Here, we show that AGE crosslinking is harnessed to activate an antibacterial phospholipase effector protein deployed by the type VI secretion system of Enterobacter cloacae. Endogenous methylglyoxal reacts with a specific arginine-lysine pair to tether the N- and C-terminal α-helices of the phospholipase domain. Substitutions at these positions abrogate both crosslinking and toxic phospholipase activity, but in vitro enzyme function can be restored with an engineered disulfide that covalently links the N- and C-termini. Thus, AGE crosslinking serves as a bona fide post-translation modification to stabilize phospholipase structure.

The crystal structure also reveals an unusual interaction between the positively charged sidechains of lipase residues Arg180 from helix α1 and Lys461 in helix α13. Fo-Fc difference maps show continuous electron density between these sidechains, suggesting that the residues are covalently linked. The +36 Da mass shift observed in the modified lipase domain is consistent with a methylglyoxal-derived imidazolium crosslink (MODIC), and MODIC fits well into the electron density bridging Arg180 and Lys461. MODIC density is also apparent in the crystal structure of chymotrypsin digested lipase•∆ss-Tli complex. In the latter structure, chymotrypsin has removed the entire catalytic core of the lipase domain (His340 - Leu445), yet helix α13 remains tethered to α1 via MODIC. Thus, AGE crosslinking joins the N- and C-termini of the lipase domain into a topological circle. This intramolecular crosslink explains increased gel mobility because the lipase cannot be denatured into a fully extended polypeptide and therefore adopts a more compact hydrodynamic radius during electrophoresis.

>MDLKPDNYFSGQQLTLARAIENGEVDEVIKLASGTDLNKPGKEDMTLLFWAVMNSINNQKTPERLNVITMLIKAGADPLQPRPQGKNSPAEFVLMADNADWIKAMLNAGLSPNAVDKTFGKPIIFQTLEAKNTKTLQAMLDKGADINITDSLGNTLLIDALDFHSYDHVLLLLERGADPEIKADNGWTMGNQLQRFLDRAKVGSDEYKKLNEIKDVLIQHGGKWPPTPVK[2x];>[2x]MAKSHHHHHHTSTKAERWQARKDLIAKGSNSLYPDAQIAAKRLAANNIAVEKAKLAENVYKTVNPLEATPGVPEGWKDISNDAGALKKYGLDKEVLFDHADTPDFLARVYQPDSAVFGSDMNPTIVFRGSRQPEFFPTKNMADWINNGAQGLGMESDYYKRAVRLGSRLAKSVSKIDIAGHSLGGGLASATSIASGQAGWTFNAAGLHSTTVEKYGGSLLGEADNIQAYRVEGELLTKIQEVNLAEDYKMLKGHIPTLIAKEEISAIMPNAAGVVHDLPGGTGGPLDRHGIGQAIDCIEQQKDEDISIIRSRA N-{3-[(4aS,7aS)-2-amino-4a,5-dihydro-4H-furo[3,4-d][1,3]thiazin-7a(7H)-yl]-4-fluorophenyl}-5-fluoropyridine-2-carboxamide 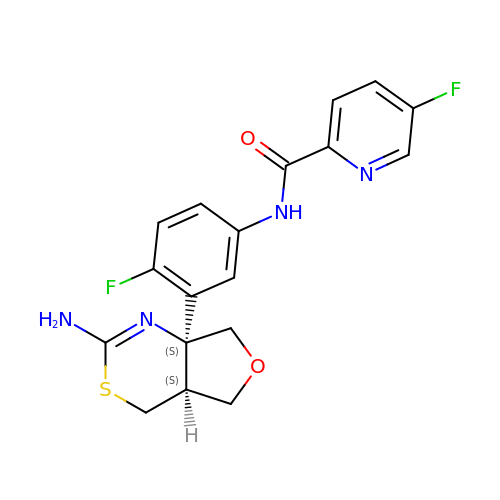| C18 H16 F2 N4 O2 S | NIDRNVHMMDAAIK-YPMLDQLKSA-N(5-thiophen-2-ylisoxazol-3-yl)methanol | C8 H7 N O2 S | 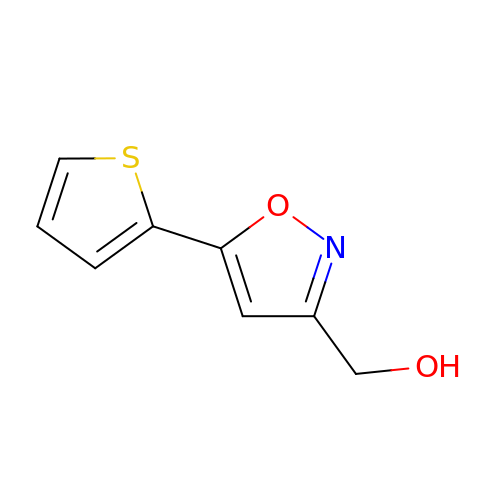HUAGDHXVPCSWLD-UHFFFAOYSA-N> RR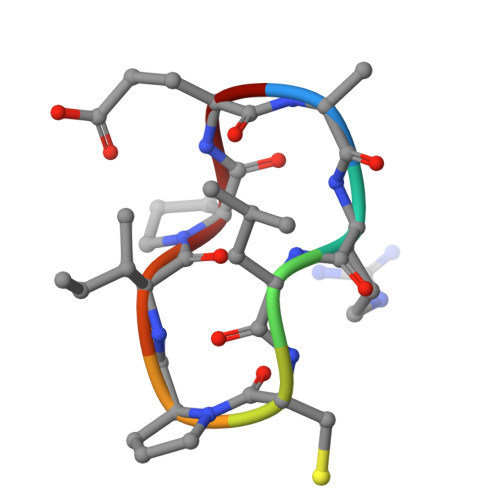LCPIPE2-[4-[[(1~{R},2~{R},6~{S},8~{R})-2-[3-[(4-ethynylphenyl)amino]-3-oxidanylidene-propyl]-9,9-dimethyl-4-azatricyclo[6.1.1.0^{2,6}]decan-4-yl]sulfonyl]phenyl]-2-methyl-propanoic 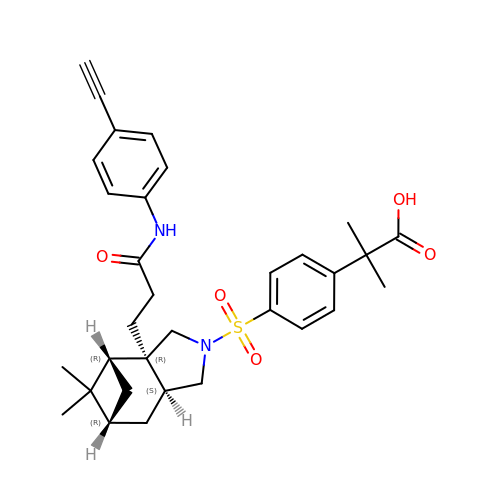acid | C32 H38 N2 O5 S | LBJWBBFBJNACAW-JSUFTFRXSA-N(3S)-3-HYDROXYHEPTANEDIOIC 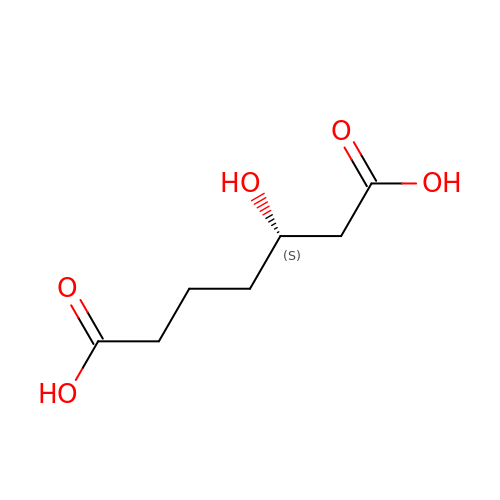ACID | C7 H12 O5 | LUQDBMUJZYJYMT-YFKPBYRVSA-N> MRRRIPSRTPGSGAKQKSWFPRRSLQVLLSAGMLSGLLGTPAALAAEPAPLPANVRADIVGYWETGGAGLKAAAEQALLGGDEAIRKFLADAPSIQHDDNRIDAARMAMTGGSGLRQAAKDAIRLSPAELEKFLLYGYEEPLDDDHKVEIARLINLGGPGVREAGKAALQGTAEERELFLNSGQYTAQQDDNRVDVARLATTGGPNVQAAAKVALRGTPEDMVEFLEVGQFTARNRDQEHATIAELIKQAELAGKQADDARKTAEESSKKAVDASQLAKEAAQKAAEETEAAKDDSQKAAVKAKQAADAARAAADAAQEAIGSANAANRAARRAALAAAQTASAATAAAEAANKAYKAAIAAAGDEGKADEAKEAAKQARAAADAATKSGLAAENAGLASAAAATASTAAKSASSNARAAAGAAEEANQHADAAGVHSNEAALAAAEARRHADAADRAADRSSALAQRAATAAYGARDAANSAAEHANKAADYADESAAHAGDSAAYAATAKRNAQAAQEAAKTATAAVTKANEIFKLARETETANLETRTDAAIERARSMKSASETSITASATTQVEALALNDTATELAKEASRPDIDVQATAAKGRQLAMQAMKLLGPWHQEAAARALSGTDQDVLDYLRTRWKEANHNDIRQQIVDLSTQSPYASVRTAAAEALNGTPEQIEAFHTTGQYTAGSDDMKVDVARLANTGGPGVSQAAKTALADGTGKTLATFLQIGQYGERLSDEKVVTARLAETGSPEVQAAAKIALAGPPELLHEFVTTGQYMAKRKDDLADVHVNQVERLLAEGSLIAAEANEDAWRATEAAATAEGAAADAATAAEKAEASAAQAKQHAADADASADAATRSAADAAASAATARDAADRAAQDATAAENSAAEAAFSAAYARDSASKADDAADRARASALAAGKSADEAEAEAKEAWKTTRALAEKEAEEARRKAAEERKRQQEQAGEPKRVCIPHPTRETMIPIMPCAASPDDSMIMPGPVDPTIRAVVWELAGLNDIKACIDKPLSGNCVMAVVGVTPWGKFKLVSKLGNGLDAVKDARGARRTVACLTGAAHSFPAGTRVLMADGTRRSIEQIEAGDLVTATDPTTGETGARTVTRTIHTPDDRNFTDVALADGSTLTSTTHHPYWSQNDQTWKNAGDLEAGDTLRTPQNTAVVIAATHDWPGLQDAYDLTVDGFHSYYVSTGTTDVLVHNNDNPCPDWVSKAWKKLPKRKSGDPTSGYVFEADGTLVWDSVLTSGRSPLSEDISAFLKGSPDFPNFPGYADVAHHAEAKIAWEMRTKMGKGKKLHIVINTNYVCPKVSSPNSMGCKQAVPAILYEDQTLYVHYPGASDALELKGTAKR;> MANTSRTRQALMAIAVSV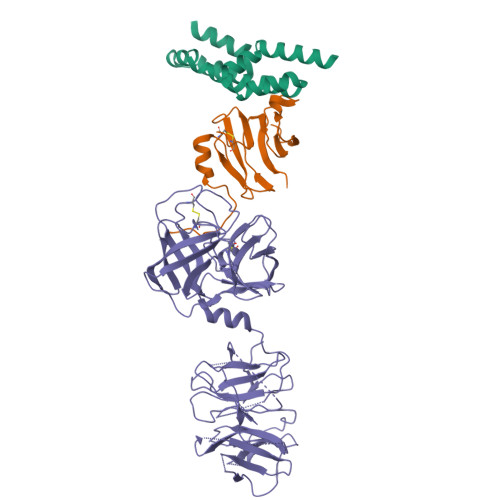LAAGVTTLGVAHADNGDAVAAAAEMPQAVEDFSYPGAAKIQAETGAILKRGNGHMLMTSCDGSEDIQVMSRTGQKDFCFNVMAKPAYLTLEVPQAYGIWTSADPVKTTIKDTDGTATVINAPANDFTGYGEAGSTGEPTTLIELRVAG;> MFRMPRPIRATALSAAVLAGALASTPAQATVGDPTTDAKLDFTARLTIGTDYRSCSGALVDTQWVLTAASCFADDPNQPDTVAAGKPAQLTRATVGRADSNIANGYVREVVELVPHPERDMVLARLDKAIPDIAPVRLASDAPTAGTPLTAVGFGRTKDEWVPIQRHQGAFTVTSVTAGAVNVTGQGGDAICAGDTGGPLLQDKNGTLHLVGVNNRSMQGGCYGSETTSTDAIAAMSDADFVTQTVNRDLGTGNLSDLVASADFNSDGRTDVAAVLEDGSLHAFYAKPDGTLEYGRELWNDNTWSPMVQIIGGDFNSDGNGDIAAVRSDGTLNLYTGTATGILNKSKPMWHDTSWKTIKQVTRFKFNGRDGLVAQWGDGNLYGYYTGTDGTLTGTKVKMWPDATWGKTRLTGTADINADGRDDLTAVRDDGSLNWYAGNTKGGLDAARKLWPDNTWTPMKRIIGGDFNGDNKGDIAAVGGQSTLLLYTGTGTGTLNKGIAMRPASGSHHHHHHHH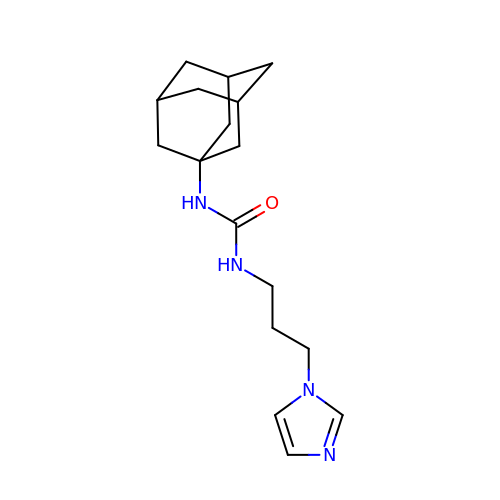1-(1-adamantyl)-3-(3-imidazol-1-ylpropyl)urea | C17 H26 N4 O | JODLYBRKXRTSIK-LTBQPASTSA-N N-undecanoyl-L-histidyl-L-histidyl-N-methyl-N-(2-pyridin-2-ylethyl)-L-tyrosinamide | C40 H55 N9 O5 | 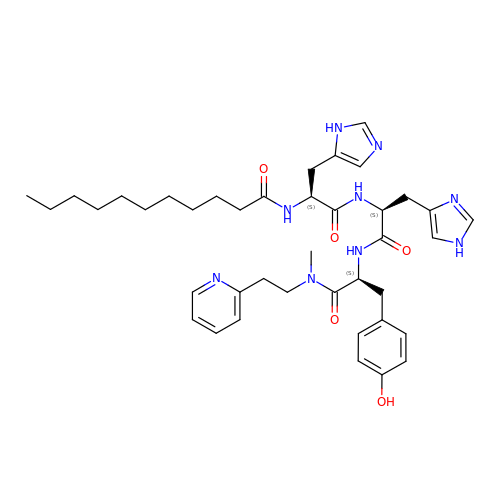XTWPUBVVNIJMOQ-KVBYWJEESA-N> MGSSKPLKGFVICCTSIDLKQRTEISTKATKLGAAYRSDFTKDVTHLIAGDFDTPKYKFAAKSRPDIKIMSSEWIPVLYESWVQGEDLDDGLLVDKHFLP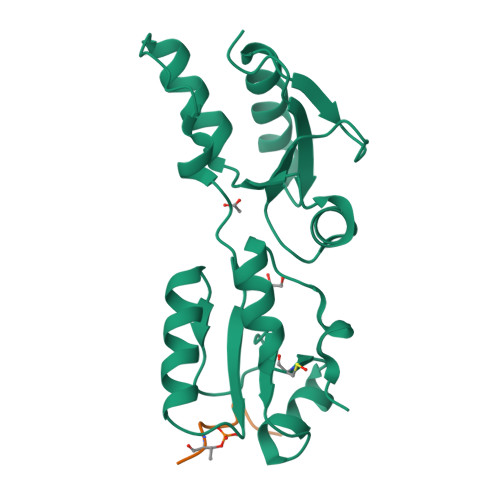TLFKCRVCLTNIGQPERSRIENYVLKHGGTFCPDLTRDVTHLIAGTSSGRKYEYALKWKINVVCVEWLWQSIQRNAVLEPQYFQLD;> GVMTVPNTPQKPNLQ>YALTEGEDYLVLDKPIPQEQSGKIEVLEFFGYFCVHCHHFDPLLLKLGKALPSDAYLRTEHVVWQPEMLGLARMAAAVNLSGLKYQANPAVFKAVYEQKIRLENRSVAGKWALSQKGFDGKKLMRAYDSPEAAAAALKMQKLTEQYRID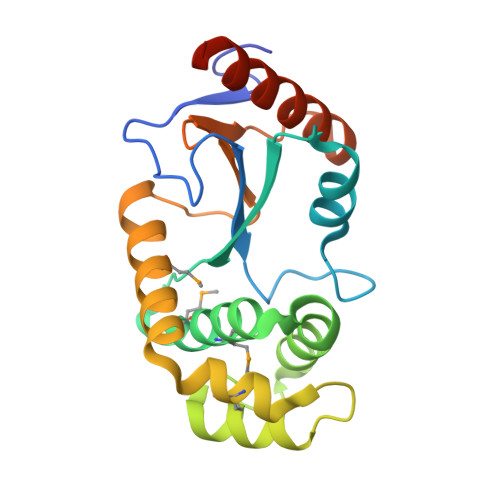STPTVIVGGKYRVIFNNGFDGGVHTIKELVAKVREERKRQTPAVQK[4x]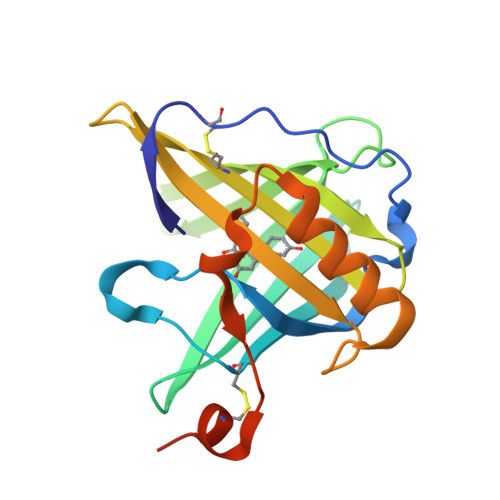>[2x]DVYHDGACPEVKPVDNFDWSQYHGKWWEVAKYPSPNGKYGKCGWAEYTPEGKSVKVSRYDVIHGKEYFMEGTAYPVGDSKIGKIYHSRTVGGYTRKTVFNVLSTDNKNYIIGYSCRYDEDKKGHWDHVWVLSRSMVLTGEAKTAVENYLIGSPVVDSQKLVYSDFSEAACKVNNSNWSHPQFEK The production of thiamine pyrophosphate (TPP), catalyzed by TPK, is critical for both catabolic and anabolic cellular processes. In yeast, this thiamine phosphate is then hydrolyzed into thiamine before pyrophosphorylation by the TPK that catalyzes the transfer of a pyrophosphate (PPi) from ATP to thiamine, resulting in AMP and TPP. CA1462 is a homodimer, with each monomer constituted of two domains.

While we did not get crystals of the TPK/Thiamine/AMP-CPP complex, the TPK incubated with thiamine and AMP-PNP produced usable crystals. However, the structure revealed that instead of a TPK/Thiamine/AMP-PNP complex, we obtained an unexpected TPK/thiamine-PNP complex with a TPNP molecule in the enzyme binding site. This result is consistent with the earlier suggestion that the pyrophosphate group is transferred at once from the ATP molecule to the thiamine moiety. The nitrogen N3 in the TPNP molecule is symmetrically opposed to its equivalent oxygen O3 in the TPP molecule. It is stabilized by a weak electrostatic interaction (3.28 Å) with the S301B γ-oxygen in the C. albicans TPK/TPNP complex. Three magnesium ions are stabilized in the active site. The first two ions superimpose exactly with the ones co-crystallised in the C. albicans TPK structure with thiamine. The third magnesium ion is coordinated by the δ-oxygen from D113 and D115 and one oxygen atom from each phosphate group of the thiamine-PNP. The last coordination of this Mg2+ involves an oxygen atom from the free inorganic phosphate symmetrically positioned with regard to the AMP phosphate shown in the mouse ATP binding site (Mg2+ number 3). The equivalent glutamine (Q206A) adopts the same conformation in the C. albicans TPK/thiamine complex and an opened conformation in the C. albicans TPK/TPNP complex. The structure containing thiamine only exhibits the closed conformation, while both are present in the TPK/TPNP complex.

>[2x]MAHHHHHHGHHHQLSEDSELIEQVIEQPDSLIISPPSDSSSSSYNHIQPFVYLESTATTQTNHNVLLILNQKITIDLISLWKKCEIIVCADGGANSLYEYFNDNNHHHHHENLQRSDYIPDYIVGDFDSISPDVKTYYESHGSKIIRQSSQYYNDFTKSIHCIQLHYQLNHTKENWFESIDEVDGLAKLWNGLNNSSDVVVDIDITIYVLNAIGGRFDQTVQSINQLYIMNEDYPKVTVFFITTNDIIFLLKKGVNYISYKNRLMFHKDNGSSPTPTCGLLPLSNKTPIILNSYGLKYDMRNWKTEMLGQVSSSNRISGETGFIVECSDDIVMNIEIDVQLDGDLEAA>[2x]MGDKPIWEQIGSSFINHYYQLFDNDRTQLGAIYIDASCLTWEGQQFQGKAAIVEKLSSLPFQKIQHSITAQDHQPTPDSCI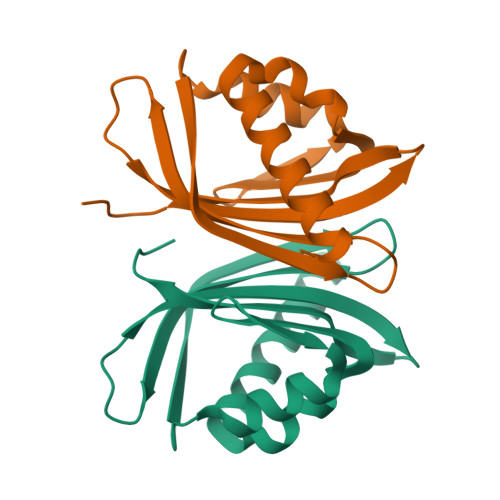ISEVVGQLKADEDPIMGFHQMFLLKNINDAWVCTNDMFRLALHNFG>[2x]MSDDFLWFEGIAFPTMGFRSETLRKVRDEFVIRDEDVIILTYPKSGTNWLAEILCLMHSKGDAKWIQSVPIWERSPWVESEIGYTALSETESPRLFSSHLPIQLFPKSFFSSKAKVIYLMRNPRDVLVSGYFFWKNMKFIKKPKSWEEYFEWFCQGTVLYGSWFDHIHGWMPMREEKNFLLLSYEELKQDTGRTIEKICQFLGKTLEPEELNLILKNSSFQSMKENKMSNYSGGSVDYVVDKAQLLRKGV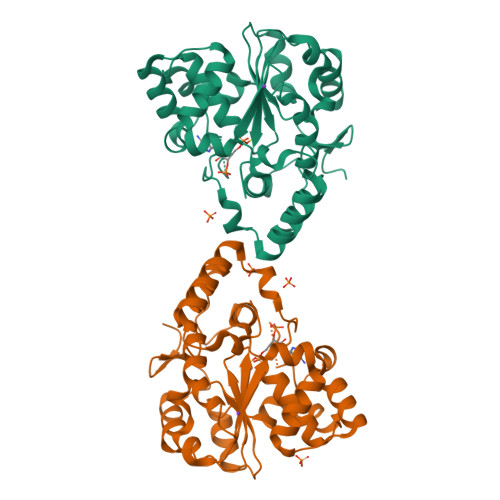SGDWKNHFTVAQAEDFDKLFQEKMADLPRELFPWE> MTSKLAVALLAAFLISAALCEGAVLPRSAKELR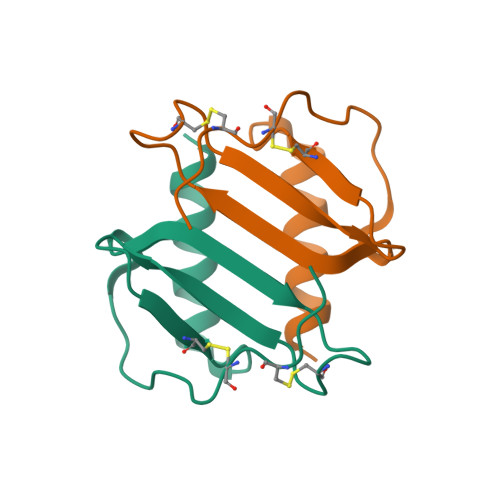CQCIKTYSKPFHPKFIKELRVIESGPHCANTEIIVKLSDGRELCLDPKENWVQRVVEKFLKRAENS The Mpp10 complex, consisting of the long disordered protein Mpp10, the uS4-like factor Imp3, and the Brix-domain protein Imp4 was identified at the center of the 90S pre-ribosome adjacent to the UTP-B module and close to the 5’ region of the U3 snoRNA. Mpp10, and its bona fide binding partners Imp3 and Imp4 have been shown to be involved in chaperoning U3::pre-18S rRNA hybrid formation by destabilization of the intramolecular box A/A’ helix of the U3 snoRNA and stabilization of the U3-hybridized state. The heterotrimeric Mpp10-Imp3-Imp4 complex is an essential 90S module, which is localized at the core of the 90S pre-ribosome adjacent to the UTP-B complex. We propose that Mpp10, positioned at the 90S core, provides an assembly scaffold with linear interaction motifs for the different members of this pentameric module.

We reconstituted a minimal complex of ctImp4 (residues 75–274) and ctMpp10 (residues 433–562) and determined its crystal structure to a resolution of 1.88 Å. Residues 433–474 as well as 506–514 of ctMpp10 are not resolved in the crystal structure. The final structure contains one ctImp4-ctMpp10 complex in the asymmetric unit. The overall fold of the ctImp4-ctMpp10 complex is very similar to that of Rpf2-Rrs1 from Aspergillus nidulans (an) and Saccharomyces cerevisiae (sc), despite the rather low sequence identity of ~17%. CtImp4 exhibits the typical BRIX fold, comprised of two anti-codon binding domains, of which one is completed by the brix-ligand, by an α-helix provided by the brix-ligand, ctMpp10 in this case. This helix contains several conserved charged (Glu536, Glue542 and Arg548) as well as hydrophobic residues (Ile545 and Ile549). Furthermore, there is no beta-augmentation on the C-terminal subdomain of ctImp4 as observed in Rpf2-Rrs1, limiting the domain complementation to helix α2. A striking difference to the Rpf2-Rrs1 complex is the presence of a long α-helix (α1) at the N-terminus of our ctMpp10 construct, which interacts via a tryptophan residue (Trp500) with ctImp4 at the interface between the two subdomains of ctImp4 (inset). While the completed Brix domain results in an excellent fit to the density, there is no corresponding density for helix α1 of ctMpp10 in any of the 90S pre-ribosomal particles. A tryptophan (Trp282) residue at the very C-terminus of ctImp4 would locate to the same position as the tryptophan of helix α1 of ctMpp10, suggesting that the current conformation may be the result of truncation and crystal packing.

> MDEYSELSGIVDPRVLVTTSRDPSSRLMAFSKEIRLMFPTAIRLNRGNLILPDLVMSAQRERLSDIILLHEHRGTPTAITISHFPHGPTLMASLHNVVLRADIPKSIKGTVSESYPHLIFEGFRTPLGQRVVKILKHLFPPRDPTNNAKSGNRVITFVNQDDCIEVRHHVYVRTNYNSVELSEVGPRFTMRPFSITMGTLE;> MDADVERAEQDVRRDLFDDLSEHEDSEDALSDASAGDPKSRKSAHERRQAKIAEQIRKLEAELVAKRAWTLAGEATAADRPVNSLLGEDMEFDHVGKPVPVVTEEVSESIEELIKRRILAGEFDEVLRRRP> IRVFAIPPSFASIFLTKSTKLTCLVTDLTTYDSVTISWTRQNGEAVKTHTNISESHPNATFSAVGEASICEDDWNSGERFTCTVTHTDLPSPLKQTISRPKGVALHRPDVYLLPPAREQLNLRESATITCLVTGFSPADVFVQWMQRGQPLSPEKYVTSAPMPEPQAPGRYFAHSILTVSEEEWNTGETYTCVVAHEALPNRVTERTVDK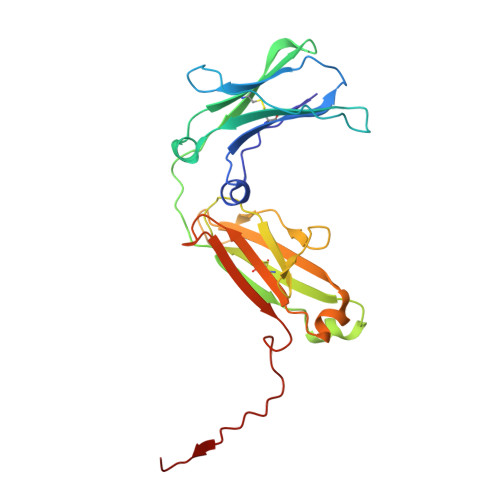STGKPTLYNVSLVMSDTAGTC>[2x]MAADISESSGADCKGDPRNSAKLDADYPLRVL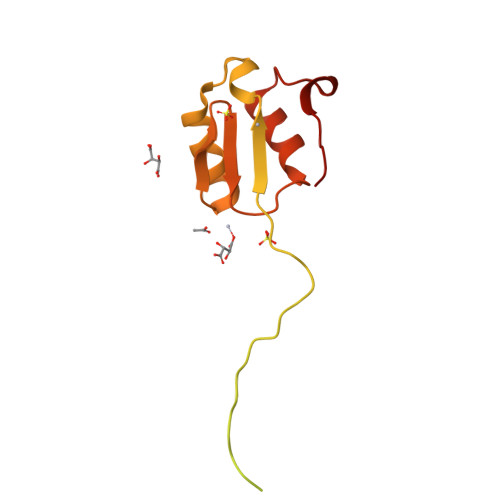YCGVCSLPTEYCEYMPDVAKCRQWLEKNFPNEFAKLTVENSPKQEAGISEGQGTAGEEEEKKKQKRGGRGQIKQKKKTVPQKVTIAKIPRAKKKYVTRVCGLATFEIDLKEAQRFFAQKFSCGASVTGEDEIIIQGDFTDDIIDVIQEKWPEVDDDSIEDLGEVKK> QSEEYCASAWVGIDGDTCETAILQTGVDFCYEDGQTSYDAWYEWYPDYAYDFSDITISEGDSIKVTVEATSKSSGSATVENLTTGQSVTHTFSGNVEGDLCETNAEWIVEDFE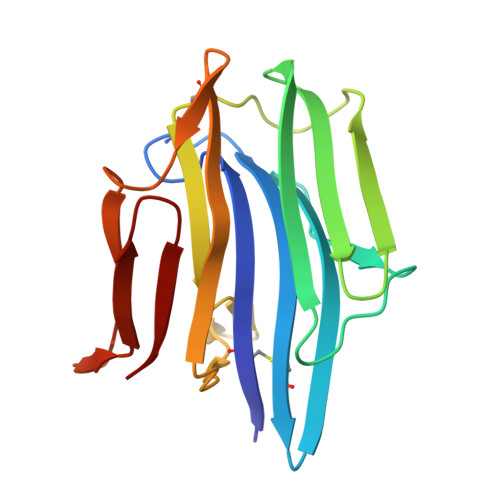SGDSLVAFADFGSVTFTNAEATSGGSTVGPSDATVMDIEQDGSVLTETSVSGDSVTVTYV> SNIYAPLYAPFFGFAGCAAAMVLSCLGAAIGTAKSGIGIAGIGTFKPELIMKSLIPVVMSGILAIYGLVVAVLIAGNLSPTEDYTLFNGFMHLSC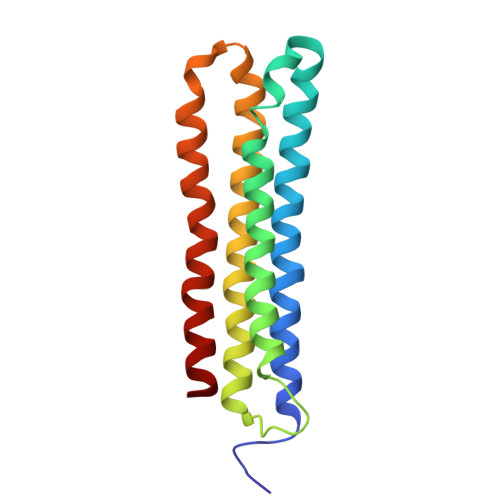GLCVGFACLSSGYAIGMVGDVGVRKYMHQPRLFVGIVLILIFSEVLGLYGMIVALILNTRGSE(5R)-3,3,5-trimethyl-5-[(1-phenyl-1H-1,2,3-triazol-4-yl)methyl]pyrrolidine-2,4-dione | C16 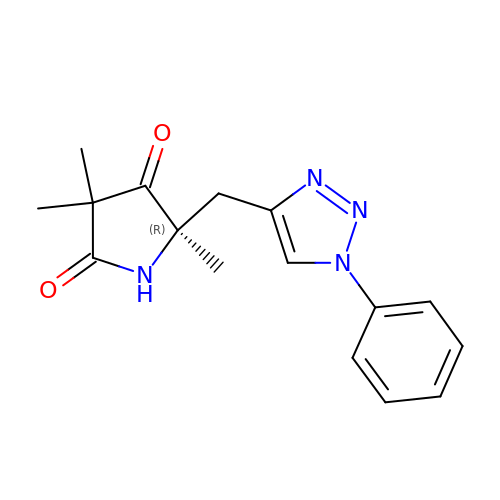H18 N4 O2 | ZHXFDNRJCWLCGX-MRXNPFEDSA-N> SLRKQRFMQFSSLEHEGEYYMTPRDFLFSVMFEQMERKTSVKKLTKKDIEDTLSGIQTAGCGSTFFRDLGDKGLISYTEYLFLLTILTKPHSGFHVAFKMLDTDGNEMIEKREFFKLQKIISKQDDLMTVKTNETGYQEAIVKEPEINTTLQMRFFGKRGQRKLHYKEFRRFMENLQTEIQEMEFLQFSKGLSFMRKEDFAEWLLFFTNTENKDIYWKNVREKLSAGESISLDEFKSFCHFTTHLEDFAIAMQMFSLAHRPVRLAEFKRAVKVATGQELSNNILDTVFKIFDLDGDECLSHEEFLGVLKNRMHRGLWVPQHQSIQEYWKCVKKES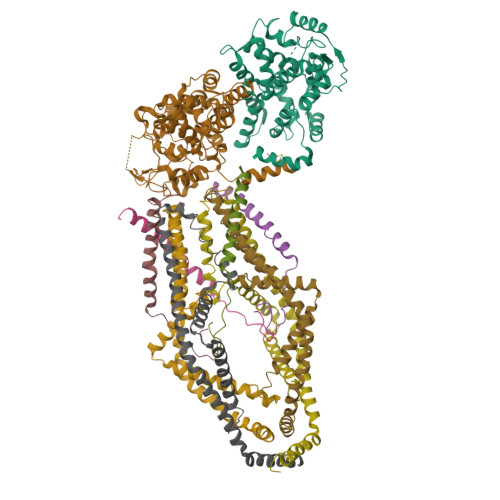;> SGFRDRKVMEYENRIRAYSTPDKIFRYFATLKVISEPGEAEVFMTPEDFVRSITPNEKQPEHLGLDQYIIKRFDGKKISQEREKFADEGSIFYTLGECGLISFSDYIFLTTVLSTPQRNFEIAFKMFDLNGDGEVDMEEFEQVQSIIRSQTSMGMRHRDRPTTGNTLKSGLCSALTTYFFGADLKGKLTIKNFLEFQRKLQHDVLKLEFERHDPVDGRITERQFGGMLLAYSGVQSKKLTAMQRQLKKHFKEGKGLTFQEVENFFTFLKNINDVDTALSFYHMAGASLDKVTMQQVARTVAKVELSDHVCDVVFALFDCDGNGELSNKEFVSIMKQRLMRGLEKPKDMGFTRLMQAMWKCAQE;>[4x]SHENAATLNDVKTLVQQLYTTLCIEQHQLNKERELIERLEDLKEQLAPLEKVRIEISRKAEKRTTLVLWGGLAYMATQFGILARLTWWEYSWDIMEPVTYFITYGSAMAMYAYFVMTRQEYVYPEARDRQYLLFFHKGAKKSRFDLEKYNQLKDAIAQAEMDLKRLRDPLQVHLPLRQ;>[4x]VIVTRSGAILPKPVKMSFGLLRVFSIVIPFLYVGTLISKNFAALLEEHDIF> GPASSNLIKQLQERGLVAQVTDEEALAERLAQGPIALYCGFDPTADSLHAGHLVPLLCLKRFQQAGHKPVALVGGATGLIGDPSFKAAERKLNTEETVQEWVDKIRKQVAPFLDFDCGENSAIAANNYDWFGNMNVLTFLRDIGKHFSVNQMINKEAVKQRLNREDQGISFTEFSYNLLQGYDFACLNKQYGVVLQIGGSDQWGNITSGIDLTRRLHQNQVFGLTVPLITKADGTKAGKTEGGAVWLDPKKTSPYKFYQFAINAADADVYRWLKFGTFMSIEEINALEEEDKNSGKA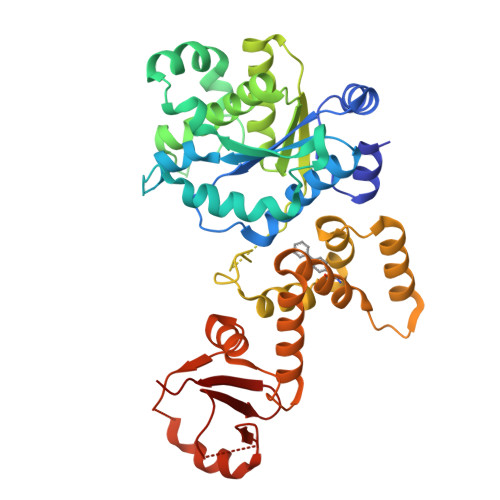PRAQYVFAEQVTRLVHGEEGLQAAKRITECLFSGSLSALSEADFEQLAQDGVPMVEMEXXXXXXXXXXXXXXXXXRLFGRFTLLRRGKKNYCLICWK>[2x]GTQSTHESLKPQRVQFQSRNFHNILQWQPGRALTGNSSVY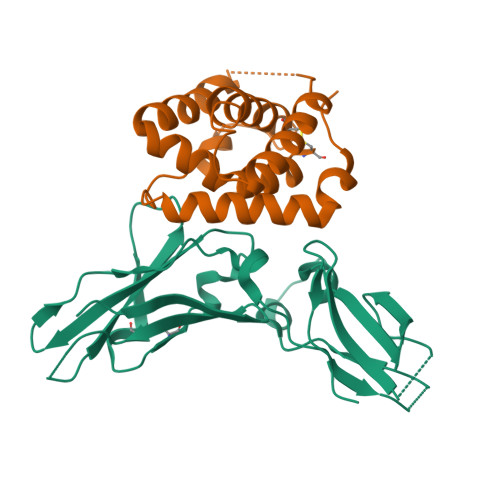FVQYKIYGQRQWKNKEDCWGTQELSCDLTSETSDIQEPYYGRVRAASAGSYSEWSMTPRFTPWWETKIDPPVMNITQVNGSLLVILHAPNLPYRYQKEKNVSIEDYYELLYRVFIINNSLEKEQKVYEGAHRAVEIEALTPHSSYCVVAEIYQPMLDRRSQRSEERCVEIP;>QGGAAAPISSHCRLDKSNFQQPYITNRTFMLAKEASLADNNTDVRLIGEKLFHGVSMSERCYLMKQVLNFTLEEVLFPQSDRFQPYMQEVVPFLARLSNRLSTCHIEGDDLHIQRNVQKLKDTVKKLGESGEIKAIGELDLLFMSLRNACI[2x]> GSHMWSQNDAMAFGSQALATAFNLDFVHYRSQISSLSPRFSDEGFAGYVNALQASNILET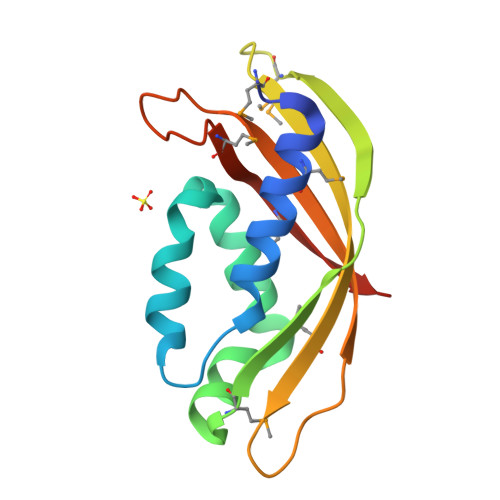IKKEKMNLTATTGAGVLVRQGQMSDGVWFWTFQYPVRMRLVGQTTSKPEQSFVFEITIQRVDPRLKPSGMEIRQMISRNAGPNS> GTHSLKYVYTGVSRGIDFPEFTAVGMVDDGQFMYFDSNSMKAVPKTEWIRQNEGADYWDRQTQVLIGAHQVFKDSIQIVMERFNQSKGVHTWQNMYGCELNDDGTTQGFYQYAYDGEDFVSLDKNTLTWTAANPQAVITKHKWEALAVAEQNKGYLENTCIEWLKKYVAYGKDTLERKVSPQVSLLQKDPSSPVTCHATGFYPSGVTITWQKNGQDHDEDVDLGELLPNEDGSFQ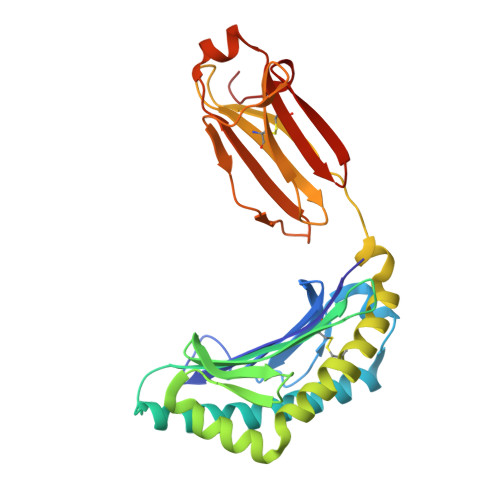RMSTLNVGPDEWKNNRFSCVVEHQDKTIRKTEDDIITNFD>APQQINDIVHRTITPLIEQQKIPGMAVAVIYQGKPYYFTWGYADIAKKQPVTQQTLFELGDVSKTFTGVLGGDAIARGEIKLSDPTTKYWPELTAKQWNGITLLHLATYTAGGLPLQVPDEVKSSSDLLRFYQNWQPAWAPGTQRLYANSSIGLFGALAVKPSGLSFEQAMQTRVFQPLKLNHTWINVPPAEEKNYAWGYREGKAVHVSPGALDAEAYGVKSTIEDMARWVQSNLKPLDINEKTLQQGIQLAQSRYWQTGDMYQGLGWEMLDWPVNPDSIINGSDNKIALAARPVKAITPPTPAVRASWVH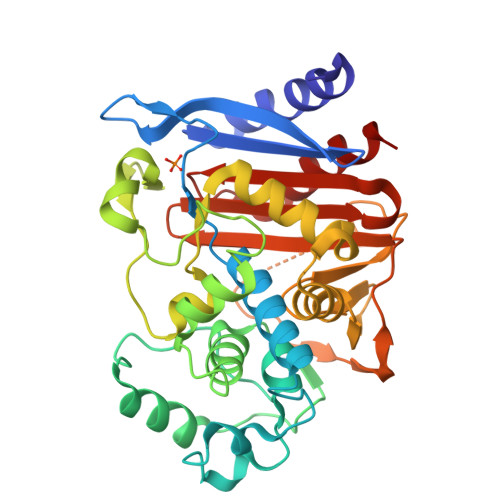KTGATGGFGSYVAFIPEKELGIVMLANKNYPNPARVDAAWQILNALQ[2x]There, 10–30% of total Cbls are bound to transcobalamin (TC). Cellular uptake of Cbls occurs via receptor-mediated endocytosis of holo-TC by means of the receptor CD320. TC consist of two domains (alpha and beta) that are connected by a flexible linker. Both domains contribute to Cbl binding, resulting in sub-pico-molar affinity.

To address the question of how Cbl mediated TC assembly proceeds, we determined crystal structures of apo TC-beta and TC-beta in complex with Cbl, putatively representing the first steps of TC assembly. We expressed the two domains of TC individually in insect cells, which lowered the affinity for Cbls while retaining the structural integrity of the domains, as no denaturing was required to generate the Cbl-free domains. After proteolytic cleavage of the MBP and further affinity purification we obtained pure, substrate free TC-beta. We next determined the crystal structure of apo TC-beta at 1.57 Å resolution, which represents to our knowledge the first structure of TC resembling a putative partial apo state of TC in the apo form (i.e. TC-alpha and TC-beta are not associated with each other). The structure was highly similar to the Cbl bound state of TC-beta (rmsd = 0.41 Å for 97 Cα-atoms), with minor changes evident in several side chains compared to CNCbl-bound TC-beta. The structures of apo TC-beta and CNCbl-bound TC-beta provide insight into distinct states of holo-TC assembly. They demonstrate the structural integrity of apo TC-beta and Cbl-bound TC-beta and therefore further consolidate the hypothesized mechanism of Cbl dependent holo-TC assembly. Virtually no structural changes occur in TC-beta upon Cbl binding, arguing against an induced fit mechanism with regards to this domain of TC. Lastly, we demonstrated that the production of apo TC-beta is a robust method to probe the interaction of TC with alternative substrates, as it is easy to produce and to co-crystallize with various substrates.

> GVDHMQTQEIISVTLQVLSLLPPYRQSISVLAGSTVEDVLKKAHELGGFTYETQASLSGPYLTSVMGKAAGEREFWQLLRDPNTPLLQGIADYRPKDGETIELRLVSW>MAQQTPLYEQHTLCGARMVDFHGWMMPLHYGSQIDEHHAVRTDAGMFDVSHMTIVDLRGSRTREFLRYLLANDVAKLTKSGKALYSGMLNASGGVIDDLIVYYFTEDFFRLVVNSATREKDLSWITQHAEPFGIEITVRDDLSMIAVQGPNAQAKAATLFNDAQRQAVEGMKPFFGVQAGDLFIATTGYTGEAGYEIALPNEKAADFWRALVEAGVKPCGLGARDTLRLEAGMNLYGQEMDETISPLAANMGWTIAWEPADRDFIGREALEVQREHGTEKLVGLVMTEKGVLRNELPVRFTDAQGNQHEGIITSGTFSPTLGYSIALARVPEGIGETAIVQIRNREMPVKVTKPVFVRNGKAVA[4x];>[2x]MSNVPAELKYSKEHEWLRKEADGTYTVGITEHAQELLG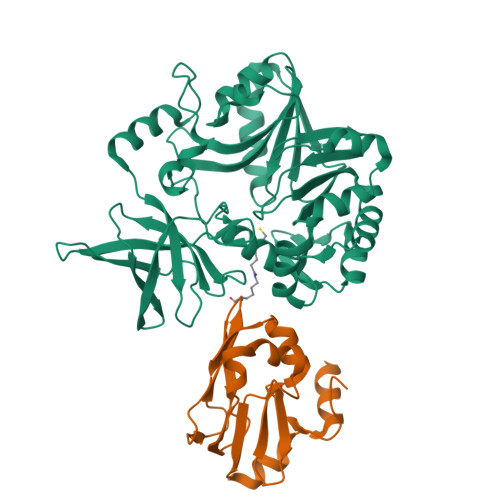DMVFVDLPEVGATVSAGDDCAVAESVKAASDIYAPVSGEIVAVNDALSDSPELVNSEPYAGGWIFKIKASDESELESLLDATAYEALLEDE>SSLPLNAIEPCVICQGRPKNGCIVH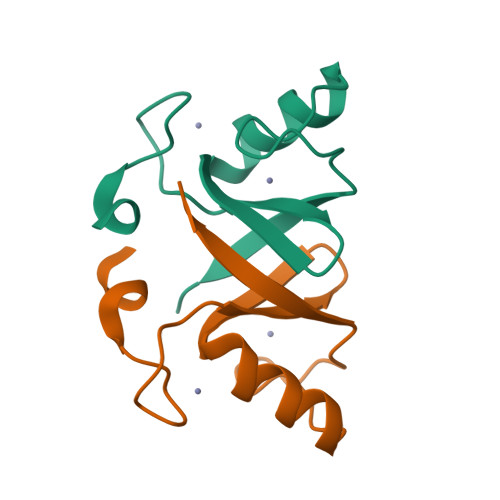GKTGHLMACFTCAKKLKKRNKPCPVCRQPIQMIVLTYFP[2x];>[2x]EDCQNLLKPCSLCEKRPRDGNIIHGRTGHLVTCFHCARRLKKAGASCPICKKEIQLVIKVFIA>MKVEEILEKALELVIPDEEEVRKGREAEEELRRRLDELGVEYVFVGSYARNTWLKGSLEIDVFLLFPEEFSKEELRERGLEIGKAVLDSYEIRYAEHPYVHGVVKGVEVDVVPCYKLKEPKNIKSAVDRTPFHHKWLEGRIKGKENEVRLLKGFLKANGIYGAEYKVRGFSGYLCELLIVFYGSFLETVKNARRWTRRTVIDVAKGEVRKGEEFFVVDPVDEKRNVAANLSLDNLARFVHLCREFMEAPSLGFFKPKHPLEIEPERLRKIVEERGTAVFAVKFRKPDIVDDNLYPQLERASRKIFEFLERENFMPLRSAFKAS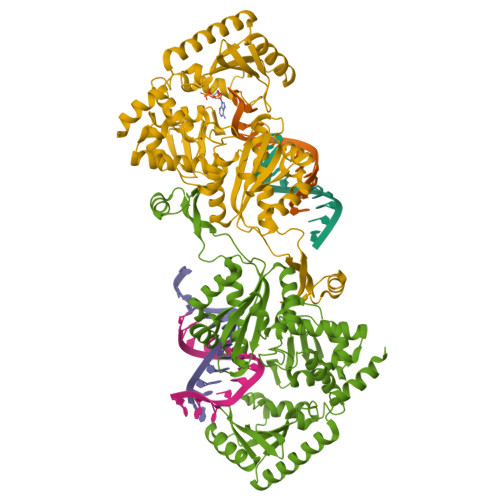EEFCYLLFECQIKEISRVFRRMGPQFEDERNVKKFLSRNRAFRPFIENGRWWAFEMRKFTTPEEGVRSYASTHWHTLGKNVGESIREYFEIISGEKLFKEPVTAELCEMMGVKD[4x]>AGHMRLTMHVPDEDMLSPLGALRLDGHFSFHDVSAMARDFGNQCSFLPAAVLHPGSVSDIAATVRHVFSLGEGSPLTVAARGHGHSLMGQSQAAQGIVVRMESLRGARLQVHDGFVDAPGGELWINVLRETLKHGLAPKSWTDYLHLTVGGTLSNAGVSGQAFRHGPQVSNVNQLEIVTGRGDVVTCSPEDNSDLFYAALGGLGQFGIITRARIALEPAPEMVRWIRVLYSDFESFTEDQEMLIMAENSFDYIEGFVIINRTGILNNWRASFKPQDPVQASHFQSDGRVLYCLELTKNFNSGDTDTMEQEVAVLLSRLRFIQSTLFHTDVTYLEFLDRVHTSELKL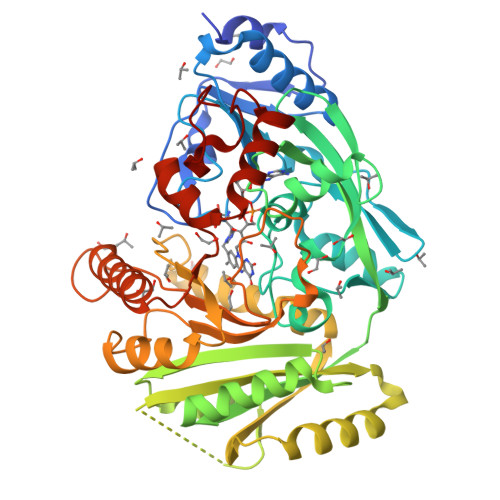RAQSLWEVPHPWLNLLIPRSSIRRFATEVFGRILKDSNNGPILLYPVNKSKWDNKTSVVIPDEEIFYLVGFLSSAPSLSGHGSIAHAMSLNSQIVEFCEEADIGMKQYLAHYTTQEQWKTHFGARWETFERRKHRYDPLAILAPGQRIFPKASLP[2x]>[6x]MSDLQKLQRFSTCDISDGLLNVYNIPTGGYFPNLTAISPPQNSSIVGTAYTVL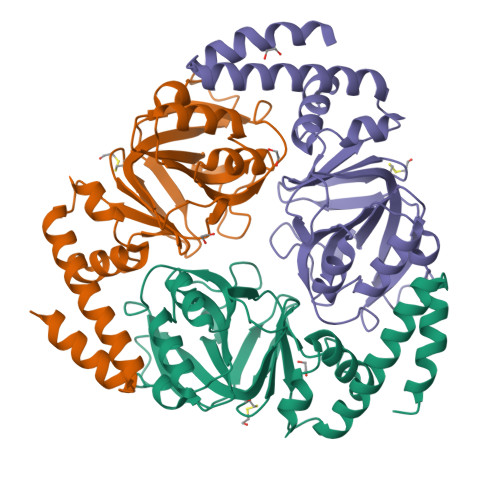FAPIDDPRPAVNYIDSVPPNSILVLALEPHLQSQFHPFIKITQAMYGGLMSTRAQYLKSNGTVVFGRIRDVDEHRTLNHPVFAYGVGSCAPKAVVKAVGTNVQLKILTSDGVTQTICPGDYIAGDNNGIVRIPVQETDISKLVTYIEKSIEVDLLVSEDIKNGIPAKQAQNDRRSVLKKYIHHHHHH>MGSSHHHHHHSSRNLYFQGGGHMFFLNLKQINDRFNTEFITKFKEILE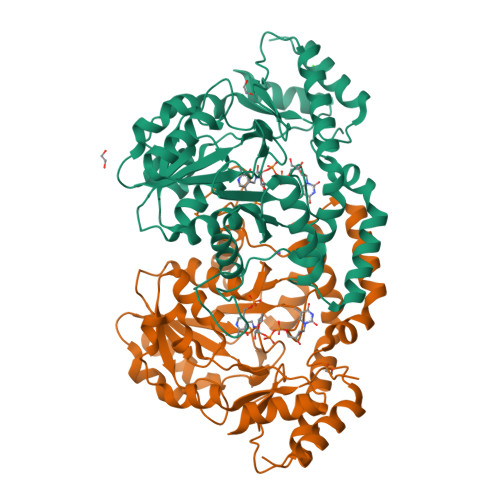SGWYILGKQCEKFENNFAKYCGVKHCIGVANGLDALRLIIKAYDFKENDEIIVPANTYIASILAITDNKCKPILIEPDINTYNINPDLIEEKITKKTKAIMVVHLYGQVCDMEKIQLLANKYNLKIIEDCAQAHGAIYKDKRVGNLGDAAGFSFYPGANLGALGDAGCICTNDDNFASKIRALANYGSHKKYENLYTGLNSRLDEIQAAFLDIKLKYLDEDNNKRKNIANFYLQNIKNENIILPSNKFDHVWHLFVVKTKLRDELQHYLNNHDIQTIIHYPIPPHKQKCYKDLNHLKLPITENIHQEVLSLPISPTMKENDFKKVADILNKWKV[4x]Interestingly, myotoxin-II (MjTX-II) isolated from Bothrops moojeni venom presents some structural differences compared to other PLA2-like proteins from the Bothrops genus. The changes in its amino acid sequence, including mutations in conserved residues (Leu32Gly and His121Tyr) and the insertion of an Asn residue at position 120, are reflected in structural changes in the hydrophobic channel and its interactions with long-chain molecules. Furthermore, fatty acids binding to MjTX-II are not necessary for the alignment of its MDoS and MDiS regions; consequently, this difference is important compared to other PLA2-like toxins, since MjTX-II activation would be facilitated. Thus, in the present work, three different techniques (myography, crystallography and bioinformatics assays) were used to test the potential inhibitory characteristics of two different ligands, acetylsalicylic acid (ASA) and rosmarinic acid (RA), against the PLA2-like myotoxin MjTX-II.

The MjTX-II/RA crystal diffracted up to 1.60 Å and belonged to the P212121 space group. The refinement converged to an Rcryst of 15.7% (Rfree = 19.1%) with one RA molecule located close to the MDiS and helix 1 from monomer A and 392 water molecules. Similar to the PrTX-I/RA complex, the crystal structure of the MjTX-II/RA complex revealed an inhibitor molecule interacting with the toxin; however, RA interacts with both monomers simultaneously and in a different region of MjTX-II. The first benzene ring region of the RA molecule (derived from the diphenyl-lactic acid portion) interacts with the N-terminus of monomer B (Asn17, Pro18 and Ala19 residues). The second benzene ring region of the RA molecule (derived from the caffeic acid portion) interacts with residues of the C-terminal region of monomer A (Leu122, Phe126 and Cys127 residues), which includes the MDiS region. RA prevented approximately 87.3% of the muscle paralysis promoted by MjTX-II in 90 minutes when both were pre-incubated (at a toxin:inhibitor ratio of 1:1, w/w., i.e., 1:40, m/m; N = 3). Several functional/structural studies with PLA2-like toxins and ligands (e.g., aristolochic and chicoric acids, suramin and Zn2+ ions)17,19,23,39 have demonstrated that their binding to the MDiS region is associated with the inhibition of these myotoxins, such as that observed in the crystal structure and functional data of the MjTX-II/RA complex presented here. The average RMS deviation of frame trajectories (ftRMSD) of the RA molecule was 0.22 ± 0.03 nm, indicating that the ligand interacts with the toxin in the same region. However, the RA effect on the MjTX-II quaternary structure results in its disturbance, forcing the toxin into a distorted conformation, evidenced by the increase of its radius of gyration (Rg) from 20.0 to 21.8 Å and COMdisp of 31.5 Å.

>SLFELGKMILQETGKNPAKSYGVYGCNCGVGGRGKPKDATDRCCYVHKCCYKKLTGCDPKKDRYSYSWKDKTIVCGENNSCLKELCECDKAVAICLRENLDTYNKKYRYNYLKPFCKKADPC[2x]> GAGCAGACATGACGTCACTCA;> ACGTCA;> TCTGAGTG;> TGTCTGC

In this work, we exhaustively probe the ability of all 36 immobile HJ sequences to form DNA crystals in two different designed systems. Three separate self-assembling DNA crystal systems are described in this report: the “4 × 5” and “4 × 6” designs (collectively referred to as the 4 × N systems), and a third construct with a “scrambled” sequence variant of the 4 × 6 lattices. Self-assembly was mediated by three constituent oligonucleotides: (S1) containing four sequence repeats of either 5 or 6 bases; (S2) composed of 21 bases containing complementary regions to both (S1); and (S3) which forms the second junction crossover. The HJ serves as the fundamental component at the core of each unit, and the ultimate assembly of the full lattice is facilitated by the complementary 2-base sticky ends that tail each duplex.

Each asymmetric unit could be defined as either a HJ containing 10 and 11 bp on each arm, or as a 21-bp linear duplex. In parallel, we employed the previously reported J1 4 × 6 system (3.05 Å), with P32 symmetry. Seventeen of the 36 junctions successfully crystallized, a 47% success rate. Unlike the 4 × 5 motif, nearly all of the 4 × 6 junction sequences had a strong preference for crystallization in buffers containing ≥2.0 M salts (e.g., LiCl, Li2SO4, KCl, and NaCl), with the majority preferring slightly basic pH conditions in cacodylic acid. The average cell constants for the P32 crystals were a = b = 68.29 Å c = 55.68 Å. However, in the majority of the crystal structures reported here, the cacodylate anion indeed fits best into the electron density map of our X-ray structures, due to the presence of sodium cacodylate in the crystallization solution.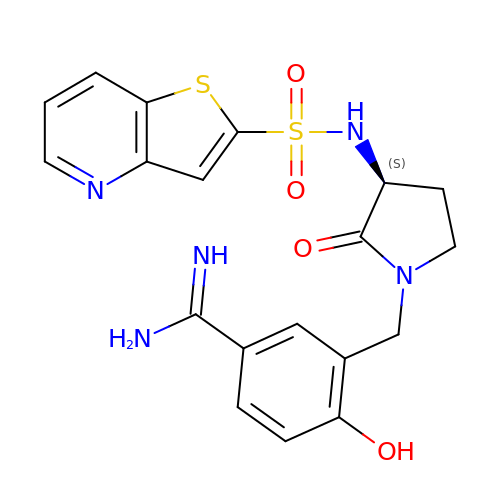4-HYDROXY-3-[2-OXO-3-(THIENO[3,2-B]PYRIDINE-2-SULFONYLAMINO)-PYRROLIDIN-1-YLMETHYL]-BENZAMIDINE | C19 H19 N5 O4 S2 | PQJGWYQPOHCEDO-ZDUSSCGKSA-N>[2x]ENSVHRYKKEASNLIKLATPVLIASVAQTGMGFVDTIMA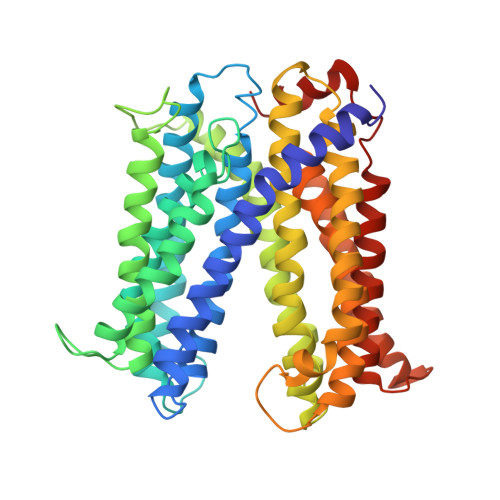GGVSAIDMAAVSIAASIWLPSILFGVGLLMALVPVVAQLNGAGRQHKIPFEVHQGLILALLVSVPIIAVLFQTQFIIRFMDVEEAMATKTVGYMHAVIFAVPAYLLFQALRSFTDGMSLTKPAMVIGFIGLLLNIPLNWIFVYGKFGAPELGGVGCGVATAIVYWIMLLLLLFYIVTSKRLAHVKVFETFHKPQPKELIRLFRLGFPVAAALFFEVTLFAVVALLVAPLGSTVVAAHQVALNFSSLVFMFPMSIGAAVSIRVGHKLGEQDTKGAAIAANVGLMTGLATACITALLTVLFREQIALLYTENQVVVALAMQLLLFAAIYQCMDAVQVVAAGSLRGYKDMTAIFHRTFISYWVLGLPTGYILGMTNWLTEQPLGAKGFWLGFIIGLSAAALMLGQRLYWLQKQSDDVQLHLAAK> GLP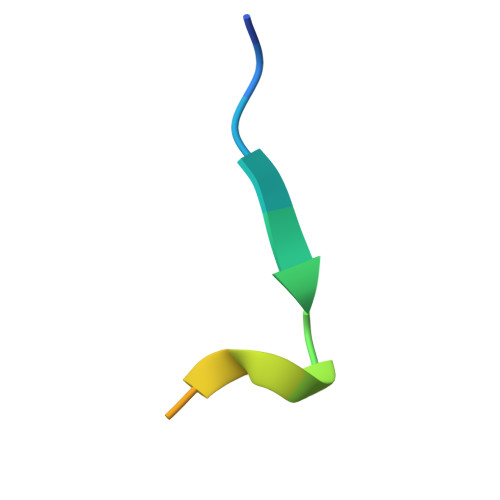VTFIDEVDSEEAPQ> MSALPEEVNRTLLQIVQAFASPDNQIRSVAEKALSEEWITENNIEYLLTFLAEQAAFSQDTTVAALSAVLFRKLALKAPITHIRKEVLAQIRSSLLKGFLSERADSIRHKLSDAIAECVQDDLPAWPELLQALIESLKSGNPNFRESSFRILTTVPYLITAVDINSILPIFQSGFTDASDNVKIAAVTAFVGYFKQLPKSEWSKLGILLPSLLNSLPRFLDDGKDDALASVFESLIELVELAPKLFKDMFDQIIQFTDMVIKNKDLEPPARTTALELLTVFSENAPQMCKSNQNYGQTLVMVTLIMMTEVSIDDDDAAEWIESDDTDDEEEVTYDHARQALDRVALKLGGEYLAAPLFQYLQQMITSTEWRERFAAMMALSSAAEGCADVLIGEIPKILDMVIPLINDPHPRVQYGCCNVLGQISTDFSPFIQRTAHDRILPALISKLTSECTSRVQTHAAAALVNFSEFASKDILEPYLDSLLTNLLVLLQSNKLYVQEQALTTIAFIAEAAKNKFIKYYDTLMPLLLNVLKVNNKDNSVLKGKCMECATLIGFAVGKEKFHEHSQELISILVALQNSDIDEDDALRSYLEQSWSRICRILGDDFVPLLPIVIPPLLITAKATQDVGLIEEEEAANFQQYPDWDVVQVQGKHIAIHTSVLDDKVSAMELLQSYATLLRGQFAVYVKEVMEEIALPSLDFYLHDGVRAAGATLIPILLSCLLAATGTQNEELVLLWHKASSKLIGGLMSEPMPEITQVYHNSLVNGIKVMGDNCLSEDQLAAFTKGVSANLTDTYERMQDRHGDGDEYNENIDEEEDFTDEDLLDEINKSIAAVLKTTNGHYLKNLENIWPMINTFLLDNEPILVIFALVVIGDLIQYGGEQTASMKNAFIPKVTECLISPDARIRQAASYIIGVCAQYAPSTYADVCIPTLDTLVQIVDFPGSKLEENRSSTENASAAIAKILYAYNSNIPNVDTYTANWFKTLPTITDKEAASFNYQFLSQ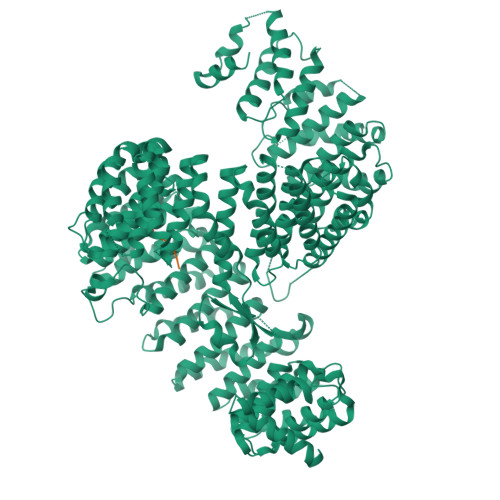LIENNSPIVCAQSNISAVVDSVIQALNERSLTEREGQTVISSVKKLLGFLPSSDAMAIFNRYPADIMEKVHKWFA;> MSVEVDKHRNTLQYHKKNPYSPLFSPISTYRCYPRVLNNPSESRRSASFSGIYKKRTNTSRFNYLNDRRVLSMEESMKDGSDRASKAGFIGGIRETLWNSGKYLWHTFVKNEPRNFDGSEVEASGNSDVESRSSGSRSSDVPYGLRENYS>[2x]SSVLASCPKKPVSSYLRFSKEQLPIFKAQNPDAKTTELIRRIAQRWRELPDSKKKIYQDAYRAEWQVYKEEISRFKEQLTPSQIMSLEKEIMDKHLKRKAMTKKKELTLLGKPKRPRSAYNVYVAERFQEAKGDSPQEKLKTVKENWKNLSDSEKELYIQHAKEDETRYHNEMKSWEEQMIEVGRKDLLRRTIKKQRKYGAEEC

Mitochondrial transcription factor A (TFAM) plays a critical role in mitochondrial transcription initiation and mitochondrial DNA (mtDNA) packaging. Both functions require DNA binding, but in one case TFAM must recognize a specific promoter sequence, while packaging requires coating of mtDNA by association with non sequence-specific regions. TFAM is composed of two tandem high-mobility group (HMG) domains connected by an α-helix linker. In this study, we identified two TFAM residues, Ser61 in HMG box1 and Pro178 in HMG box2, that form specific hydrogen bonds with N2 of two guanine bases separated by 10 nucleotides (GN10G consensus).

In order to further investigate whether the GN10G consensus could drive TFAM binding to DNA, we decided to crystallize TFAM in complex with a 22-mer nonspecific sequence (NS2) containing a single GN10G consensus where all other nucleotides were randomized with respect to the sequence used for our LSP structure. Strikingly, the TFAM-NS2 structure showed a unique arrangement. All TFAM-DNA structures determined to date have revealed that a molecule of TFAM interacts with a molecule of DNA (1:1 ratio of TFAM to DNA) (19,20,30,35). However, in the TFAM-NS2 structure, the binding site of TFAM was composed of two halves of adjacent DNA molecules. HMG box 1 of a TFAM molecule interacts with half of a DNA molecule, while HMG box 2 binds to a different DNA molecule (see scheme on Figure 5B). Intriguingly, the TFAM-NS2 structure was also bound a GN10G consensus, although in this case the consensus was formed between two adjacent DNA molecules. Since nothing in our experimental setup prevented TFAM from binding a single DNA molecule, under our experimental conditions DNA bridging appears to be preferred, although the reason for this preference is unclear. A similar structure has also been observed for Abf2p, the yeast TFAM homolog, indicating that the ability to bridge DNA ends is common to both proteins. Importantly, Abf2p plays no role in transcriptional initiation, perhaps suggesting that this ability might be relevant to the role of these proteins in mtDNA packaging.> MVAPLSVQGNKILANGQPASFSGMSLFWSNTEWGGEKYYNAQVVSWLKSDWNAKLVRAAMGVEDEGGYLTDPANKDRVTQVVDAAIANDMYVIIDWHSHNAHQYQSQAIAFFQEMARKYGANNHVIYEIYNEPLQVSWSNTIKPYAQAVIAAIRAIDPDNLIIVGTPTWSQDVDVAANDPITGYQNIAYTLHFYAGTHGQYLRDKAQTALNRGIALFVTEWGSVNANGDGAVANSETNAWVSFMKTNHISNANWALNDKVEGASALVPGASANGGWVNS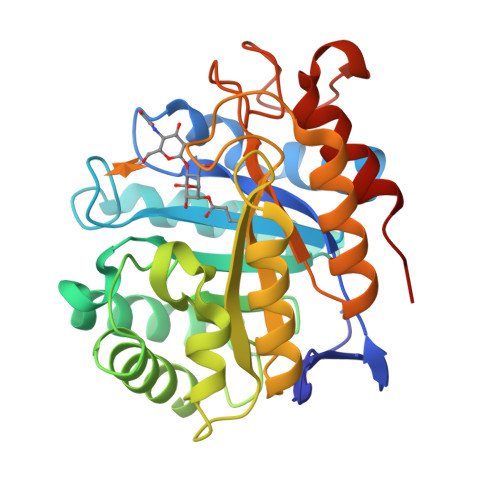QLTASGALAKSIISGWPSYLEHHHHHH>GSHADYNLNSPLISDDIDNLIRKFNSLPIPSMWDSKNWDGVLEMLTSCQANPISTSQMHKWMGSWLMSDNHDASQGYSFLHEVDKEAEITFDVVETFIRGWGNKPIEYIKKERWTDSFKILAYLCQKFLDLHKLTLILNAVSEVELLNLARTFKGKVRRSSHGTNICRIRVPSLGPTFISEGWAYFKKLDILMDRNFLLMVKDVIIGRMQTVLSMVCRIDNLFSEQDIFSLLNIYRIGDKIVERQGNFSYDLIKMVEPICNLKLMKLARESRPLVPQFPHFENHIKTSVDEGAKIDRGIRFLHDQIMSVKTVDLTLVIYGSFRHWGHPFIDYYTGLEK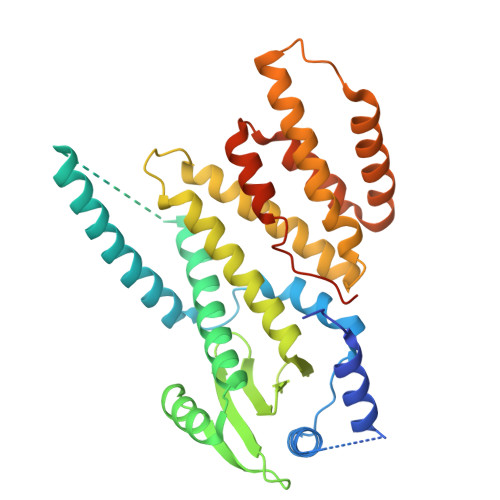LHSQVTMKK[2x]> KEGYLVNKSTGCKYGCLKLGENEGCDKECKAKNQGGSYGYCYAFACWCEGLPESTP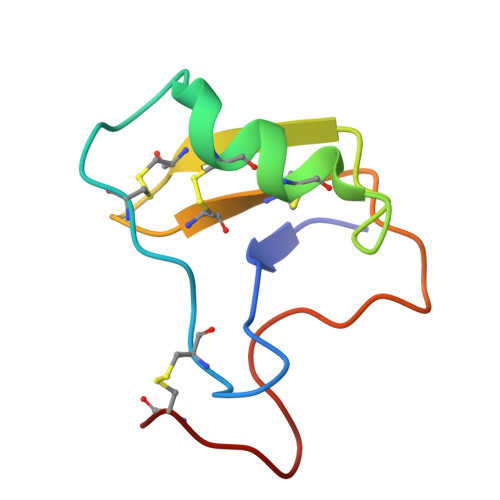TYPLPNKSCS> LLGGLPTDLVSNAGGQLFYGRPQVSENGEPSVKLYTSVEAAQLDHGVTIPHDIDLGVSAITLQDFDNQHLQDRPTPSPAPARPITNWRSGDVVWVTLPSAEYAQSQSAMGSHPAYWSEEATII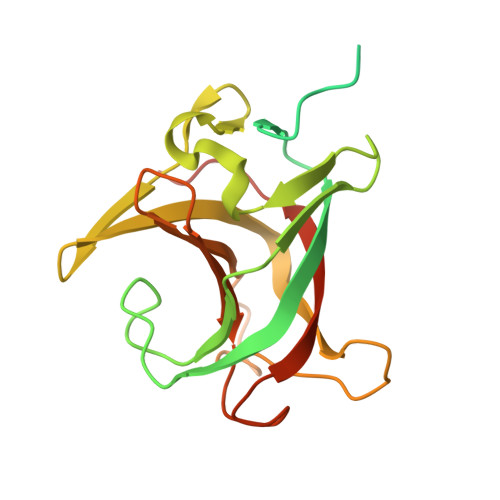NVATGQRAAVSSIKWDQVTLNGKALHKETHSGLVYYQLPLMGKINFWQQGTTKAGYTYNYNTTDSDSLWVWWDGGSKAYLYISTYTTMLGAGPVNITGLGAVGPNPVDQASAAVPM> MGSHHHHHHDITSLYKKAGSAAAVLEENLYFQGSFTMRRKVFEELVTATKILLNEGIMDTFGHISARDPEDPASFFLAQKLAPSLITVDDIQRFNLDGETSDNRPSYLERYIHSEIYKTRPDV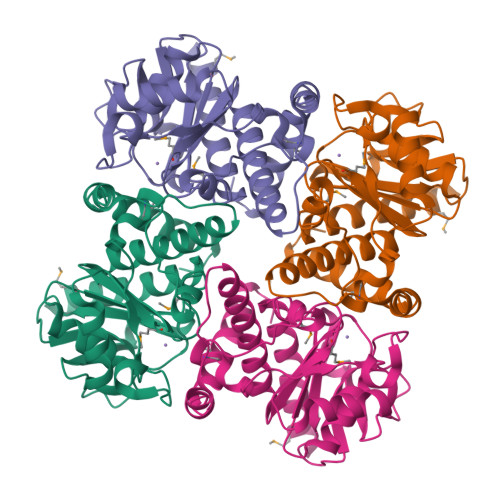QCVLHTHSPAVLPYCFVDTPLRPVTHMGAFIGESVPVYEIRDKHGDETDLFGGSPDVCADIAESLGSQTVVLMARHGVVNVGKSVREVVFRAFYLEQEAAALTAGLKIGNVKYLSPGEIKTAGKLVGAQIDRGWNHWSQRLRQAGLA> AEGKLN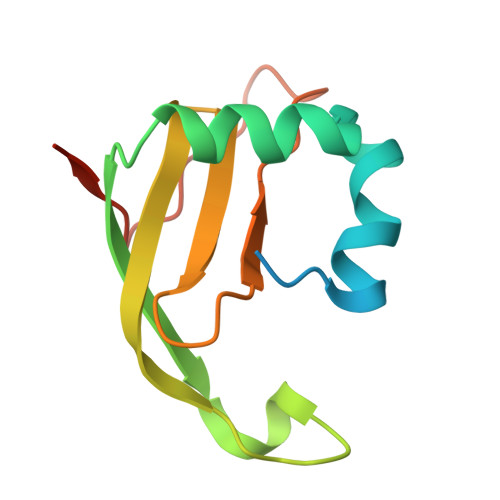DELAKNKGKIPGLKIDQKIRGQMPERGWTEDDIKNTVSNGATGTSFDKRSPKKTPPDYLGRNDPATVYGSPGKYVVVNDRTGEVTQISDKTDPGWVDDSRIQWGNKNDQ>[6x]HHHHHHMQRKNDMQTQRLRIAIQKKGRLSQECQELLKKCGVKFNIMGERLVVHSLNMPIDLLLVRDDDIPGLIMDGVVDLGFVGENVLEETRLDRL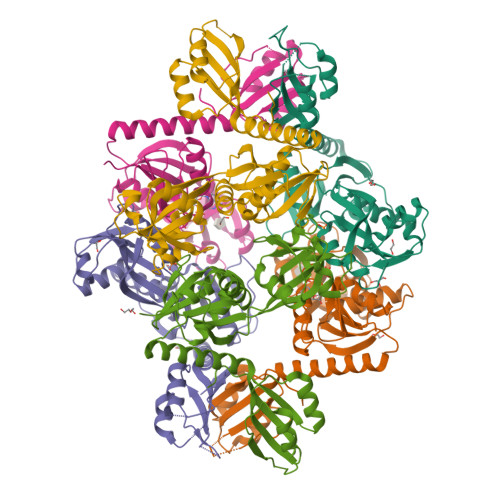ALNQRNEFTTLRRMDFGGCRLSIAIEKDAEYRGPQDLNGKRIATTYPQLLKAYMDRQGVDFSTCMLTGSVEVAPRAGLADAIADLVSTGATLEANGLKEVEVIFESKATLIQRPGAFAADKAALIDKLLTRMHGVQQAKESKYIMLHAPVEKLAQIKTLLPGAEDPTVLPLSADKSKVAVHMVSSENLFWETMEQLKALGASSILVLPIEKMME> MAAAVVLAAGLRAARRAVAATGVRGGQVRGAAGVTDGNEVAKAQQATPGGAAPTIFSRILDKSLPADILYEDQQCLV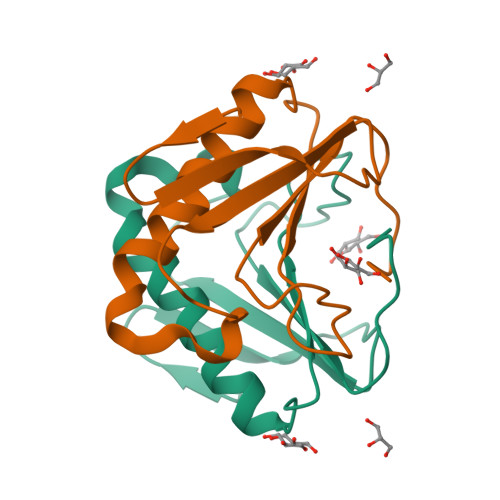FRDVAPQAPVHFLVIPKKPIPRISQAEEEDQQLLGHLLLVAKQTAKAEGLGDGYRLVINDGKLGAQSVYHLHIHVLGGRQLQWPPG> MPLDPVIQQVLDQLNRMPAPDYKHLSAQQFRSQQSLFPPVKKEPVAEVREFDMDLPGRTLKVRMYRPEGVEPPYPALVYYHGGGWVVGDLETHDPVCRVLAKDGRAVVFSVDYRLAPEHKFPAAVEDAYDALQWIAERAADFHLDPARIAVGGDSAGGNLAAVTSILAKERGGPAIAFQLLIYPSTGYDPAHPPASIE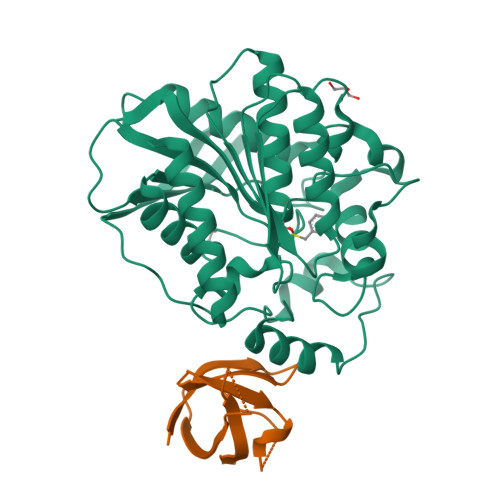ENAEGYLLTGGMMLWFRDQYLNSLEELTHPWFSPVLYPDLSGLPPAYIATAQYDPLRDVGKLYAEALNKAGVKVEIENFEDLIHGFAQFYSLSPGATKALVRIAEKLRDALA;> RGKVKWFHDYYGYGFITKDEGGDVFVNADAIDMEGFKTLKEGQVVEFEIDSTVANAPQAAHVKVVE>MRGLRKEALEELMKLLNMKDFPYRIEGIDISHLQGKYTVASLVVFEDGFPKKGDYRRYKIEQDHPDDYESIRTVVKRRYSKHPLPNLLFVDGGIGQVNAAIEALKEIGKDCPVVGLAKKEETVVFENREIHLPHD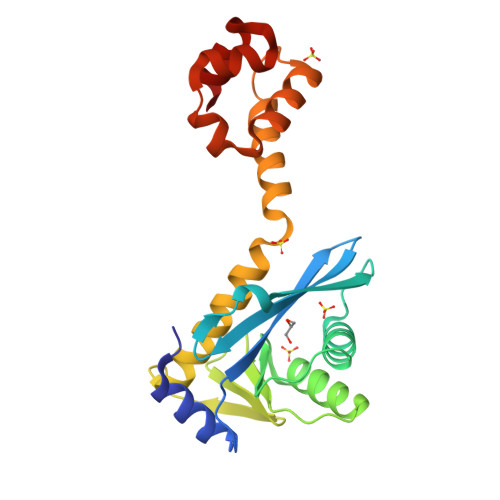HPVLRLLVQIRDETHRFAVSYHRKRREKESLRSVLDNVPGIGPIRKKKLIEHFGSLENIRSASLEEIARVIGSTEIARRVLDILG[2x]>MGHHHHHHHHHHMQSSVNEFLTPRHIDVQVVSQTRAKITLEPLERGFGHTLGNALRRILLSSMPGCAVVEAEIDGVLHEYSAIEGVQEDVIEILLNLKGLAIKLHGRDEVTLTLAKKGSGVVTAADIQLDHDVEIINGDHVIANLADNGALNMKLKVARGRGYEPADARQSDEDESRSIGRLQLDASFSPVRRVSYVVENARVEQRTNLDKLVLDLETNGTLDPEEAIRRAATILQQQLAAFVDLKGDSEPVVEEQEDEIDPILLRPVDDLELTVRSANCLKAENIYYIGDLIQRTEVELLKTPNLGKKSLTEIKDVLASRGLSLGMRLDNWPPASLKKDDKATA[2x];> MGMAYSYTEKKRIRKDFSKLPDVMDVPYLLAIQLDSYREFLQAGATKEQFRDVGLHAAFKSVFPIISYSGNAALEYVGYRLGEPAFDVKECVLRGVTFAVPLRVKVRLIIFDRESSNKAIKDIKEQEVYMGEIPLMTENGTFIINGTERVIVSQLHRSPGVFFDHDRGKTHSSGKLLYSARIIPYRGSWLDFEFDPKDCVFVRIDRRRKLPASVLLRALGYSTEEILNAFYATNVFHIKGETLNLELVPQRLRGEVASIDIKDGSGKVIVEQGRRITARHINQLEKAGVSQLEVPFDYLIGRTIAKAIVHPATGEIIAECNTELTLDLLAKVAKAQVVRIETLYTNDIDCGPFISDTLKIDNTSNQLEALVEIYRMMRPGEPPTKEAAETLFGNLFFSAERYDLSAVGRMKFNRRIGRTEIEGPGVLSKEDIIDVLKTLVDIRNGKGIVDDIDHLGNRRVRCVGEMAENQFRVGLVRVERAVKERLSMAESEGLMPQDLINAKPVAAAIKEFFGSSQLSQFMDQNNPLSEITHKRRVSALGPGGLTRERAGFEVRDVHPTHYGRVCPIETPEGPNIGLINSLATYARTNKYGFLESPYRVVKDSLVTDEIVFLSAIEEADHVIAQASATLNEKGQLVDELVAVRHLNEFTVKAPEDVTLMDVSPKQVVSVAASLIPFLEHDDANRALMGSNMQRQAVPTLRADKPLVGTGMERNVARDSGVCVVARRGGVIDSVDASRVVVRVADDEVETGEAGVDIYNLTKYTRSNQNTCINQRPLVSKGDVVARGDILADGPSTDMGELALGQNMRVAFMPWNGFNFEDSICLSERVVQEDRFTTIHIQELTCVARDTKLGPEEITADIPNVGEAALNKLDEAGIVYVGAEVQAGDILVGKVTPKGETQLTPEEKLLRAIFGEKASDVKDTSLRVPTGTKGTVIDVQVFTRDGVERDSRALSIEKMQLDQIRKDLNEEFRIVEGATFERLRAALVGAKAEGGPALKKGTEITDDYLDGLERGQWFKLRMADDALNEQLEKAQAYISDRRQLLDDKFEDKKRKLQQGDDLAPGVLKIVKVYLAIKRRIQPGDKMAGRHGNKGVVSVIMPVEDMPHDANGTPVDIVLNPLGVPSRMNVGQILETHLGLAAKGLGEKINRMLEEQRKVAELRKFLHEIYNEIGGREENLDELGDNEILALAKNLRGGVPMATPVFDGAKEREIKAMLKLADLPESGQMRLFDGRTGNQFERPTTVGYMYMLKLNHLVDDKMHARSTGSYSLVTQQPLGGKAQFGGQRFGEMEVWALEAYGAAYTLQEMLTVKSDDVNGRTKMYKNIVDGDHRMEAGMPESFNVLIKEIRSLGIDIELETE;> MLKDLLNLLKNQGQIEEFDAIRIGLASPEMIRSWSFGEVKKPETINYRTFKPERDGLFCAKIFGPVKDYECLCGKYKRLKHRGVICEKCGVEVALAKVRRERMGHIELASPVAHIWFLKSLPSRIGLLLDMTLRDIERVLYFESYVVIDPGMTTLEKGQLLNDEQYFEALEEFGDDFDARMGAEAVHELLNAIDLEHEIGRLREEIPQTNSETKIKKLSKRLKLMEAFQGSGNKPEWMVLTVLPVLPPDLRPLVPLDGGRFATSDLNDLYRRVINRNNRLKRLLDLAAPDIIVRNEKRMLQEAVDALLDNGRRGRAITGSNKRPLKSLADMIKGKQGRFRQNLLGKRVDYSGRSVITVGPTLRLHQCGLPKKMALELFKPFIFGKLEGRGMATTIKAAKKMVERELPEVWDVLAEVIREHPVLLNRAPTLHRLGIQAFEPVLIEGKAIQLHPLVCAAYNADFDGDQMAVHVPLTLEAQLEARALMMSTNNILSPANGEPIIVPSQDVVMGLYYMTREAINAKGEGMAFADLQEVDRAYRSGQASLHARVKVRINEKIKGEDGQLTANTRIVDTTVGRALLFQVVPAGLPFDVVNQSMKKKAISKLINHCYRVVGLKDTVIFADQLMYTGFAYSTISGVSIGVNDFVIPDEKARIINAATDEVKEIESQYASGLVTQGEKYNKVIDLWSKANDEVSKAMMANLSKEKVVDREGKEVDQESFNSMYMMADSGARGSAAQIRQLAGMRGLMAKPDGSIIETPITANFREGLNVLQYFISTHGARKGLADTALKTANSGYLTRRLVDVAQDLVVTEIDCGTEHGLLMSPHIEGGDVVEPLGERVLGRVIARDVFKPGSDEVIVPAGTLIDEKWVDFLEVMSVDEVVVRSPITCETRHGICAMCYGRDLARGHRVNIGEAVGVIAAQSIGEPGTQLTMRTFHIGGAASRTSAADNVQVKNGGTIRLHNLKHVVRADGALVAVSRSGELAVADDFGRERERYKLPYGAVISVKEGDKVDPGAIVAKWDPHTHPIVTEVDGTVAFVGMEEGITVKRQTDELTGLTNIEVMDPKDRPAAGKDIRPAVKLIDAAGKDLLLPGTDVPAQYFLPANALVNLTDGAKVSIGDVVARIPQETSKTRDITGGLPRVADLFEARRPKEPSILAEISGTISFGKETKGKRRLVITPNDGSDPYEELIPKWRHLNVFEGEQVNRGEVISDGPSNPHDILRLLGVSSLAKYIVNEIQDVYRLQGVKINDKHIETILRQMLRKVEVSESGDSSFIKGDQVELTQVLEENEQLGTEDKFPAKYERVLLGITKASLSTESFISAASFQETTRVLTEAAVTGKRDFLRGLKENVVVGRLIPAGTGLAYHSERKRQRDLGKPQRVSASEAEAALTEALNSSGNGSGSWSHPQFEK;> MARVTVEDCLDNVDNRFELVMLATKRARQLATGGKEPKVAWENDKPTVVALREIASGLVDENVVQQEDIVEDEPLFAAFDDEANTEAL;> MALKKEGPEFDHDDEVLLLEPGIMLDESSADEQPSPRATPKATTSFSSKQHKHIDYTRALDATQLYLNEIGFSPLLTPEEEVHFARLAQKGDPAGRKRMIESNLRLVVKIARRYVNRGLSLLDLIEEGNLGLIRAVEKFDPERGFRFSTYATWWIRQTIERAIMNQTRTIRLPIHVVKELNVYLRAARELTHKLDHEPSPEEIANLLEKPVAEVKRMLGLNERVTSVDVSLGPDSDKTLLDTLTDDRPTDPCELLQDDDLSESIDQWLTELTDKQREVVIRRFGLRGHESSTLEEVGQEIGLTRERVRQIQVEALKRLREILEKNGLSSDALFQLEHHHHHH;> GAMGMSEEELEQDELDGA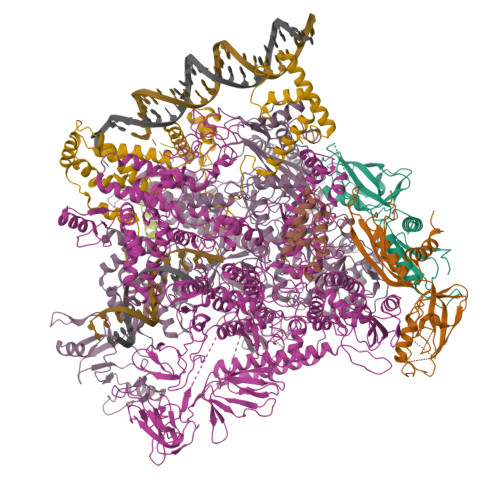DEDDGEELAAADDGEADSGDGDEAPAPGKKAKAAVVEEELPSVEAKQKERDALAKAMEEFLSRGGKVQEIEPNVVADPPKKPDSKYGSRPI>DVVPHHKLTVNNTKAMKHALERVQLPWKKHSFQEHQSVTSETNTDEHIKDIYDDTERELAFYKQSLDAVLVARDELKRLKVPFKRPLDYFAEMVKSDEHMDKIKGKLIEE[2x];>QFMNKQR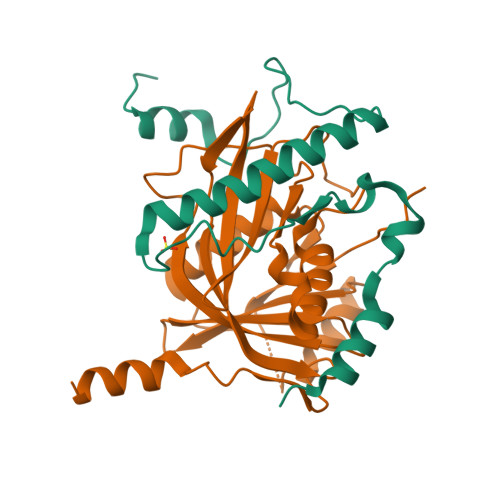TLLISSRGVNYRHRHLIQDLSGLLPHSRKEPKLDTKKDLQQLNEIAELYNCNNVLFFEARKHQDLYLWLSKPPNGPTIKFYIQNLHTMDELNFTGNCLKGSRPVLSFDQRFESSPHYQLIKELLVHNFGVPPNARKSKPFIDHVMSFSIVDDKIWVRTYEISHSTKNKEEYEDGEEDISLVEIGPRFVMTVILILEGSFGGPKIYENKQYVSPNVVRAQIKQQAAEE[2x]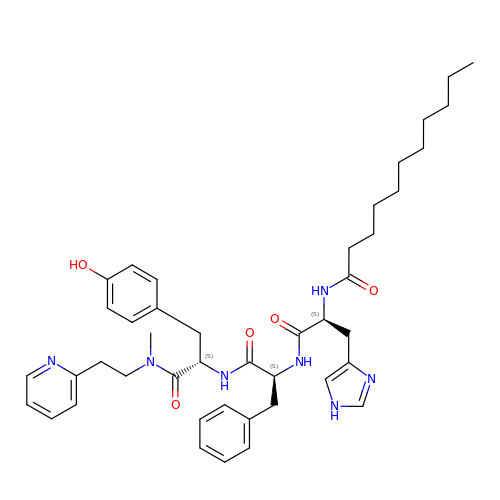N-undecanoyl-L-histidyl-L-phenylalanyl-N-methyl-N-(2-pyridin-2-ylethyl)-L-tyrosinamide | C43 H57 N7 O5 | KGRSUMUKTYCXCP-IGMOWHQGSA-N>[2x]S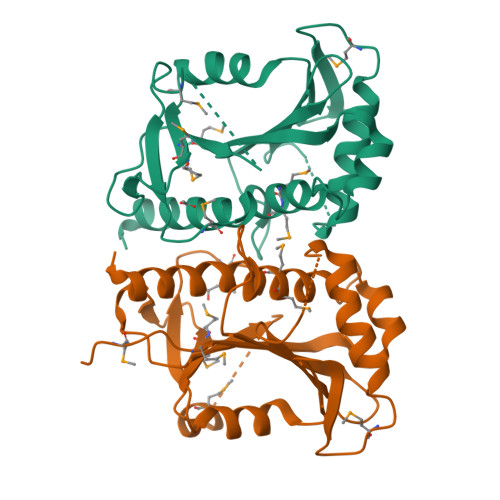NAMRNTMRSFILRARSAPTDSQRLLDEIGGKCHTEILAHCMMNSLFTAQSHREDVVIHLVLESTRDYSRTITVEANEISDVGGFHEAALIALLVKALDASVGMGKEQTRVVQPGLTVRTISFEALLGELAEHHSLYMMDKKGDSIRDIKIGPNPCFILTDHIPMPKKSGNSMKRLGVEKISLGPKMLFASQCVTLIHNEIDHQEAGW> MTHSSQRRILLLAAAAAPLALSVGACAARD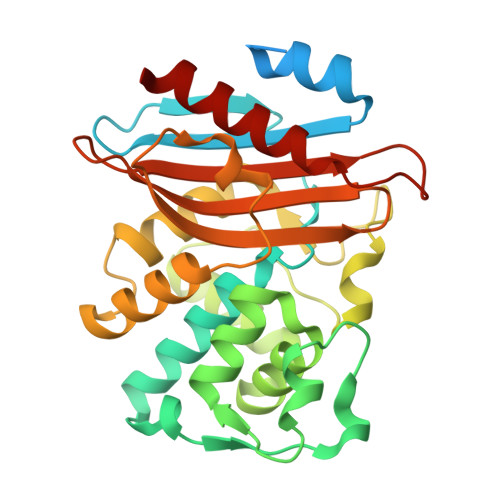AAVSDAASPVGAAPASFAALERAAGGRLGVCAIDTATGRRTLHRADERFPFCSTFKAMLGAAVLAQSVAHPGLLQQRVTYGRSDLVSYSPVTERHVDTGMTVAELCAATIQYSDSTAANELMKLIGGPAAVTAYARSIGDDTFRLDRWETELNTALPGDLRDTTTPAAMAASLRVLVLGDALPAAQRAQLIEWLRGNKVGDKRIRAGVPTGWRVGDKTGTGDYGTTNDAGVLWPPSRAPIVLAVYYTQTRADAKAKDDVIATATRIAIATLG> MALEICVKAAVGAPDHLGDCPFSQRALLTL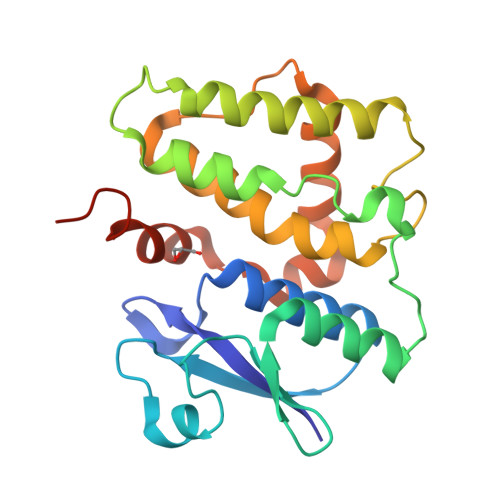EEKSLTYKIHLINLSDKPQWFLDISPQGKVPVLKIDDKWVTDSDVIVGILEEKYPDPPLKTPAEFASVGSNIFGTFGTFLKSKDSNDGSEHALLVELEALENHLKSHDGPFIAGERVSAVDLSLAPKLYHLQVALGHFKSWSVPESFPHVHNYMKTLFSLDSFEKTKTEEKYVISGWAPKVNPVEHHHHHH>[6x]ATPHINAEMGDFADVVLMPGDPLRAKYIAETFLEDAREVNNVRGMLGFTGTYKGRKISVMGHGMGIPSCSIYTKELITDFGVKKIIRVGSCGAVLPHVKLRDVVIGMGACTDSKVNRIRFKDHDFAAIADFDMVRNAVDAAKALGIDARVGNLFSADLFYSPDGEMFDVMEKYGILGVEMEAAGIYGVAAEFGAKALTICTVSAHIRTHEQTTAAEAQTTFNDMIKIALESVLLGDK

Purine nucleoside phosphorylase (PNP, purine nucleoside orthophosphate ribosyl transferase, EC 2.4.2.1) has a crucial role in the purine salvage pathway. It catalyses the reversible phosphorolytic cleavage of the glycosidic bond of purine (2′-deoxy) nucleosides, generating the corresponding free base and (2′-deoxy) ribose 1-phosphate. E. coli PNP is an excellent molecular machine conducting efficient catalysis of purine nucleosides glycosidic bond cleavage. It is a homohexamer, built as a trimer of dimers, with all its subunits having the active site in the open conformation in the apo enzyme form. Monomers in each dimer mutually donate two amino acids (His4 and Arg43) to complete their active sites.

In the case of orthorhombic structures of the wild-type enzyme with two formycin molecules (WT-6(P/S)-2FA) and of the double mutant complexes with two and four formycin molecules per hexamer bound, (DM-6(P/S)-2FA and DM-6(P/S)-4FA, respectively) all six monomers are crystallographically independent, whereas in the case of hexagonal structures of the wild-type and the mutant with six formycin molecules bound by each hexamer (WT-6(P/S)-6FA and DM-6(P/S)-6FA) two halves of the hexamer are related by the crystallographic two-fold axis. Although the active sites A and F are closed in the structure of DM-6(P/S)-2FA, these sites are not first occupied by FA molecules. The only active sites that are occupied with FA molecules in structure DM-6(P/S)-2FA are open active sites D and C from the closed-open dimer. Occupancy factor for both FA molecules in these active sites is 0.7. Closed active sites A and F and open active sites B and E are filled with water molecules only. The order of filling the active sites has changed with respect to the wild-type enzyme. It is evident that changing the two most important amino acids from the nucleoside binding site, Asp204 and Arg217, completely changed the affinity and probably cooperativity of the subunits (which is reflected in the kinetic properties ). And indeed, in the structure of the DM enzyme, active sites in the closed conformation are not the ones that are occupied first by nucleoside - open sites are those that bind nucleoside in the beginning. In the case of DM, which is not able to protonate the substrate independently of active site conformation, as Asp204 residue is missing in this enzyme form (replaced by Ala), the nucleoside is bound mostly in active sites adopting the open conformation.>GGSGGSGGMGEQPIFTTRAHVFQIDPSTKKNWVPASKQAVTVSYFYDVTRNSYRIISVDGAKVIINSTITPNMTFTKTSQKFG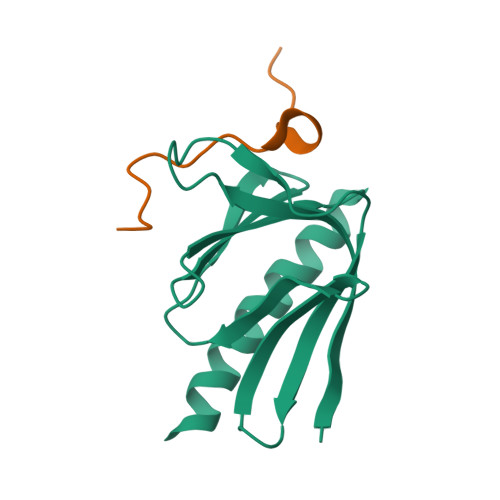QWADSRANTVFGLGFSSELQLTKFAEKFQEVREAARLARD[3x];>LLNFDELPEPPATFCDPEEVEGSGENLQ[3x]>SWMWNQFFLLEEYTGSDYQYVGKLHSDQDRGDGSLKYILSGDGAGDLFIINENTGDIQATKRLDREEKPVYILRAQAVNRRTGRPVEPESEFIIKIHDINDNEPIFTKDVYTATVPEMADVGTFVVQVTATDADDPTYGNSAKVVYSILQGQPYFSVESET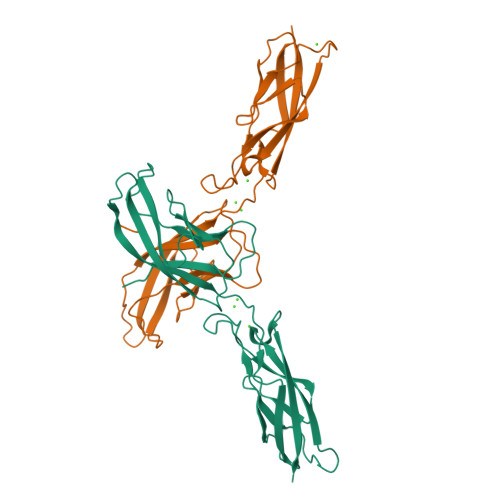GIIKTALLNMDRENREQYQVVIQAKDMGGQMGGLSGTTTVNITLTD[4x]> GSMDYKDDDDKKTNWLKRIYRVRPCVKCKVAPRNWKVKNKHLRIYNMCKTCFNNSIDIGDDTYHGH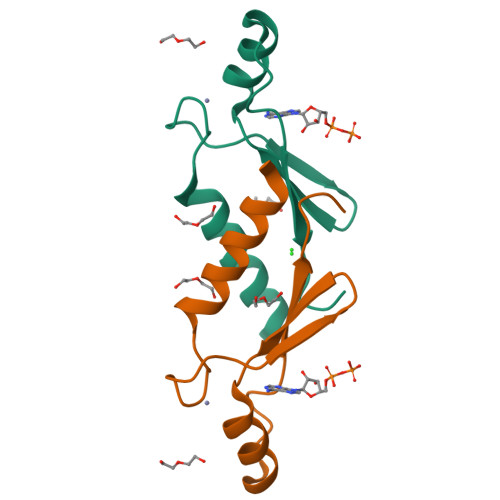VDWLMYADSKEISNT> MEPPNLYPVKLYVYDLSKGLARRLSPIMLGKQLEGIWHTSIVVHKDEFFFG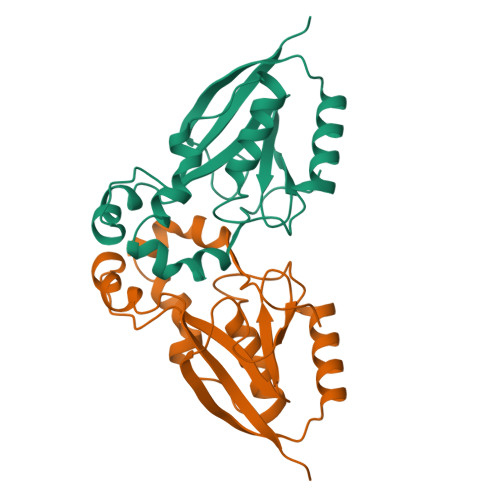SSGISSCTPGGTLLGPPDSVVDVGNTEVTEEIFLEYLSSLGESLFRGEAYNLFEHNCNTFSNEVAQFLTGRKIPSYITDLPSEVLSTPFGQALRPFLDSIQIQPPGGNSVGRPNGQS>[3x]MLQCYNCPNPTADCKTAVNCSSDFDACLITK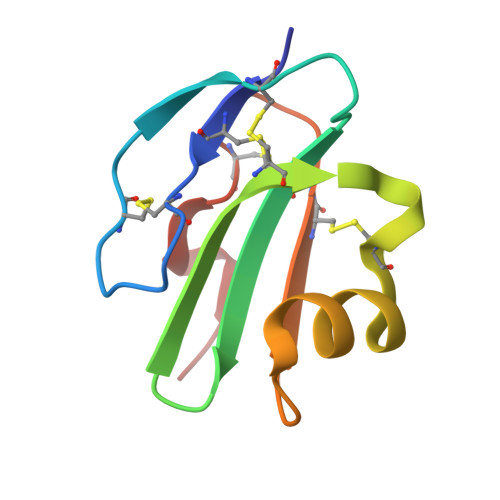AGLQVYNKCWKFEHCNFNDVTTRLRENELTYYCCKKDLCNFNEQLEN>MHDSMKAGVYEIEQGMSVRQVLEMLSDADNAQMNRVLVIEGTTFKQLITALKNDKNVKNTILDLPDDQLMKALGIPYHHPEGLFAPNTYFFAKGETDKKILTDLYHRQMKALDAAWAKRAPNLPYKDKYEALIM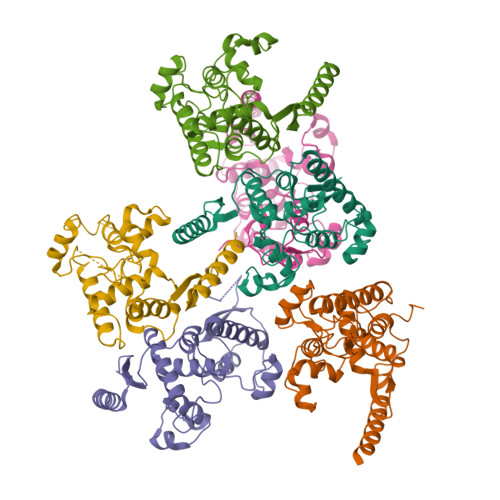ASIVEKETSLDSELTQVSGVFVRRLKLGMRLQTDPTVIYGMGANYKGNITREDLRTPTPYNTYTINGLPPTPIALPSQKAIEAALHPDDSNNIYFVATGNGGHKFTADLQAHNQAVQEYLSVLRSKKLEHHHHHH[6x]> HHHHHHEQKLISEEDLEGIKYRRNELFLDVLESVNLLMSPQGQVLSAHVSGRVVMKSYLSGMPECKFGMNDKIVIEKQGKGTADETSKSGKQSIAIDDCTFHQCVRLSKFDSERSISFIPPDGEFELMRYRTTKDIILPFRVIPLVREVGRTKLEVKVVIKSNFKPSLLAQKIEVRIPTPLNTSGVQVICMKGKAKYKASENAIVWKIKRM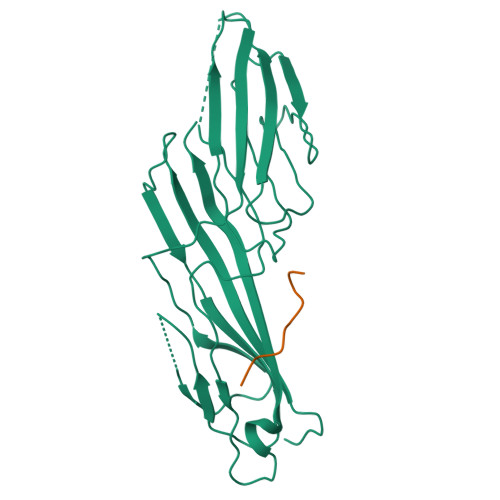AGMKESQISAEIELLPTNDKKKWARPPISMNFEVPFAPSGLKVRYLKVFEPKLNYSDHDVIKWVRYIGRSGIYETRC;> TTGVYVKMPPT> GSSAAPGAIQCMNRHKMERHGKMPAGYKGFDCNVCDQPMLKITEKAYMYRCEKCDYDVCNQCAESRKFKEVHFLCAKCGKKFPSQTKLQYHSRGCRGPS

Kinetoplastids are evolutionarily divergent eukaryotes that have an unconventional set of kinetochore proteins. In this study, we focused on KKT2 and KKT3, which are homologous to each other and have three domains conserved among kinetoplastids: A protein kinase domain classified as unique among known eukaryotic kinase subfamilies, a central domain of unknown function, and divergent polo boxes. In this report, we have revealed a unique zinc-binding domain in the KKT2 and KKT3 central domain, which is important for their kinetochore localization and function in T. brucei. In this study, we show that KKT2 and KKT3 are important for recruiting multiple kinetochore proteins, including KKT1, KKT4, KKT14, KKT22, and KKT23, while localization of KKT2 and KKT3 is independent from various kinetochore proteins. Together with the fact that KKT2 and KKT3 have DNA-binding motifs, these results support the hypothesis that KKT2 and KKT3 locate at the base of kinetoplastid kinetochores and play crucial roles in recruiting other kinetochore proteins.

We obtained crystals of BsKKT2572–668, which corresponds to residues 569–664 in T. brucei KKT2, and determined its structure to 1.8-Å resolution by zinc single-wavelength anomalous dispersion (Zn-SAD) phasing. Our analysis revealed the presence of two distinct zinc-binding domains: The N-terminal one (referred to as the CL domain for its key role in centromere localization; see below) consists of two β-sheets (where β-strands 1, 4, and 5 comprise the first β-sheet, and β-strands 2 and 3 comprise the second β-sheet) and one α-helix, while the C-terminal one consists of one β-sheet (comprising β-strands 6 and 7) and one α-helix. The CL domain coordinates two zinc ions and the C-terminal domain coordinates one zinc ion. The closest structural homologue of the BsKKT2 CL domain was the atypical C1 domain of the Vav1 protein (root mean square deviation [RMSD]: 2.7 Å across 52 Cα). Coordination of one zinc ion in the BsKKT2 CL domain occurs via the N-terminal residues Cys580 and His584, while that in the Vav1 C1 domain occurs via the N-terminal His516 and C-terminal Cys564. More importantly, the CL domain does not have the HX12CX2CXnCX2CX4HX2CX7C motif that is present in all C1 domains. Structural analysis of the C-terminal zinc-binding domain of BsKKT2 revealed a classical C2H2-type zinc finger. The C-terminal zinc-binding domain of BsKKT2 consists of one C2H2 domain (−1: Ser653; 2: Thr655; 3: Lys656; 6: Tyr659). Our analysis revealed a highly conserved acidic patch centered around residue BsKKT2 D626. The crystal structure of the B. saltans KKT2 central domain revealed a unique structure, which consists of two distinct zinc-binding domains, the CL domain and C2H2-type zinc finger.> GGGTGGGTGGGTGGGTTAGCGTTA;> TAACGC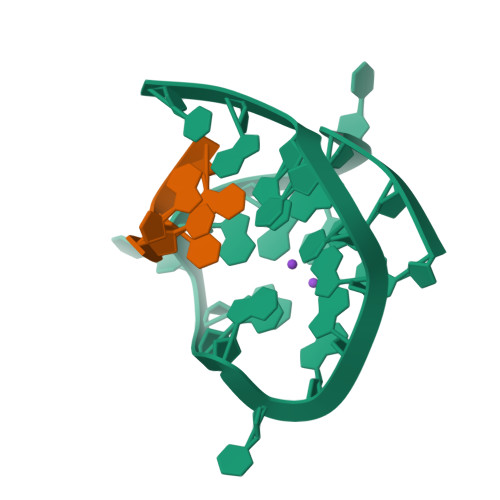TA> KL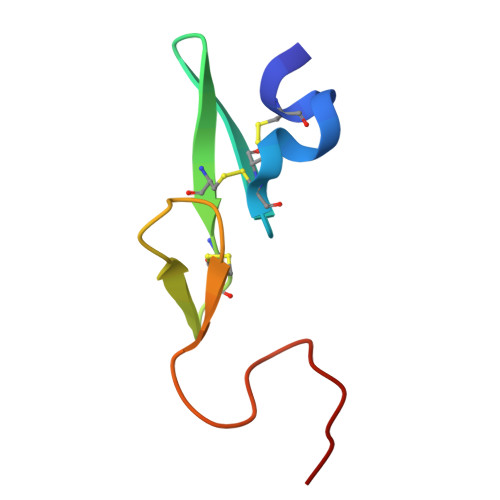CSLDNGDCDQFCHEEQNSVVCSCARGYTLADNGKACIPTGPYPCGKQTLE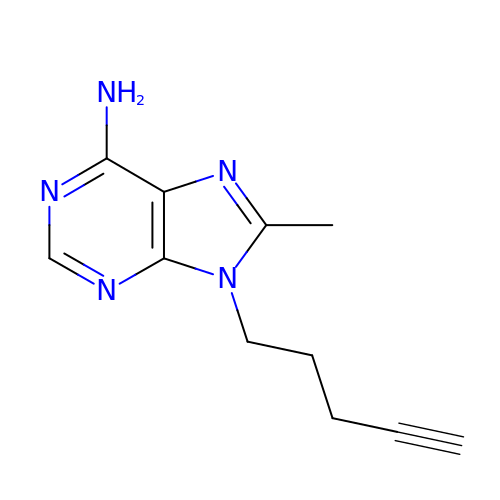8-methyl-9-pent-4-ynyl-purin-6-amine | C11 H13 N5 | XNRGOKLMAXATIA-UHFFFAOYSA-N>ANINKLYSDIDPEMKMDWNKDVSRSLGLRSIKNSLLGIITTRKGSRPFDPEFGCDLSDQLFENMTPLTADTVERNIESAVRNYEPRIDKLAVNVIPVYDDYTLIVEIRFSVIDNPDDIEQIKLQLASSNRV[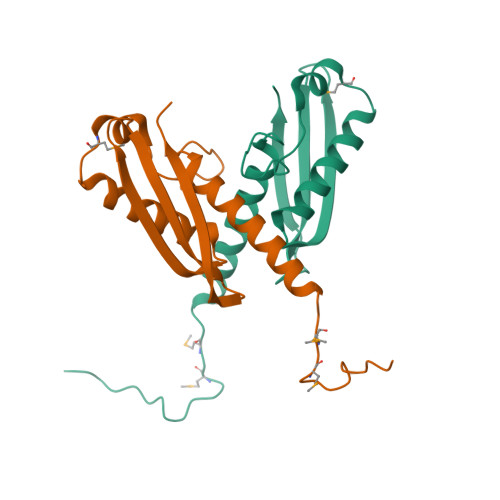2x]>[2x]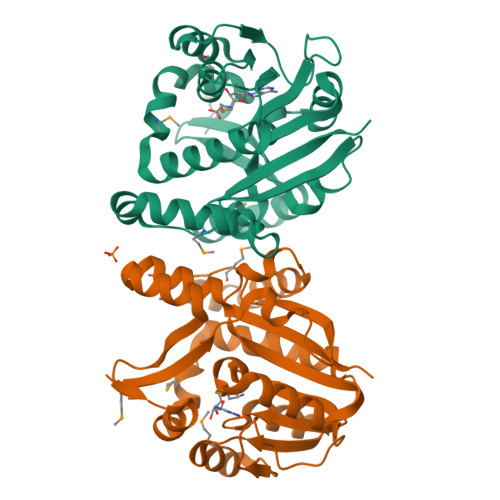MGSDKIHHHHHHMKLRSWEFYDRIARAYDSMYETPKWKLYHRLIGSFLEEYLKNPCRVLDLGGGTGKWSLFLQERGFEVVLVDPSKEMLEVAREKGVKNVVEAKAEDLPFPSGAFEAVLALGDVLSYVENKDKAFSEIRRVLVPDGLLIATVDNFYTFLQQMIEKDAWDQITRFLKTQTTSVGTTLFSFNSYAFKPEDLDSLEGFETVDIRGIGVMEYPDERISEREETIFRLEQELSRDRNIIWKADHIFFVLKKKRGA(4R,5R)-4,5,6-tris(oxidanyl)-2-oxidanylidene-hexanoic acid | C6 H10 O6 | 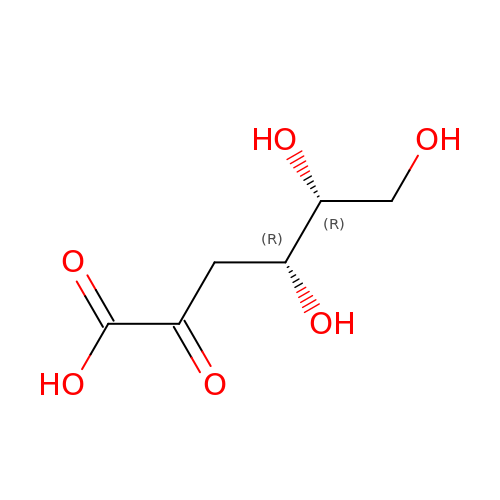WPAMZTWLKIDIOP-NQXXGFSBSA-N>[4x]GSHMSQKFDVVVIGAGPGGYVAAIRAAQLGLKTACIEKYIGKEGKVALGGTCLNVGCIPSKALLDSSYKYHEAKEAFKVHGIEAKGVTIDVPAMVARKANIVKNLTGGIATLFKANGVTSFEGHGKLL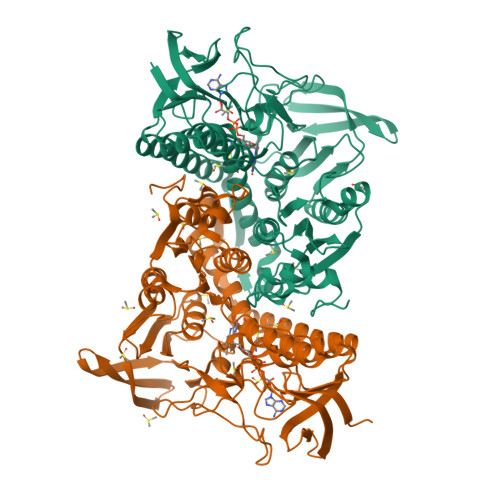ANKQVEVTGLDGKTQVLEAENVIIASGSRPVEIPPAPLTDDIIVDSTGALEFQAVPKKLGVIGAGVIGLELGSVWARLGAEVTVLEALDKFLPAADEQIAKEALKVLTKQGLNIRLGARVTASEVKKKQVTVTFTDANGEQKETFDKLIVAVGRRPVTTDLLAADSGVTLDERGFIYVDDHCKTSVPGVFAIGDVVRGAMLAHKASEEGVMVAERIAGHKAQMNYDLIPSVIYTHPEIAWVGKTEQTLKAEGVEVNVGTFPFAASGRAMAANDTTGLVKVIADAKTDRVLGVHVIGPSAAELVQQGAIGMEFGTSAEDLGMMVFSHPTLSEALHEAALAVNGHAIHIANRKKR>MVPISPIETVPVKLKPGMDGPKVKQWPLTEEKIKALVEICTEMEKEGKISKIGPENPYNTPVFAIKKKDSTKWRKLVDFRELNKRTQDFWEVQLGIPHPAGLKKKKSVTVLDVGDAYFSVPLDEDFRKYTAFTIPSINNETPGIRYQYNVLPQGWKGSPAIFQSSMTKILEPFKKQNPDIVIYQYMDDLYVGSDLEIGQHRTKIEELRQHLLRWGLTTPDKKHQKEPPFLWMGYELHPDKWTVQPIVLPEKDSWTVNDIQKLVGKLNWASQIYPGIKVRQLCKLLRGTKALTEVIPLTEEAELELAENREILKEPVHGVYYDPSKDLIAEIQKQGQGQWTYQIYQEPFKNLKTGKYARMRGAHTNDVKQLTEAVQKITTESIVIWGKTPKFKLPIQKETWETWWTEYWQATWIPEWEFVNTPPLVKLWYQLEKEPIVGAETFYVDGAANRE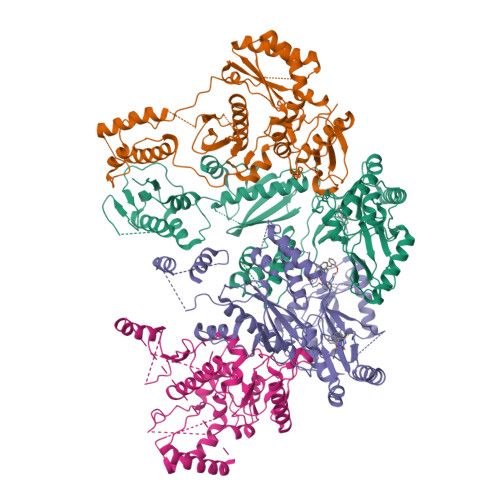TKLGKAGYVTNKGRQKVVPLTNTTNQKTELQAIYLALQDSGLEVNIVTDSQYALGIIQAQPDKSESELVNQIIEQLIKKEKVYLAWVPAHKGIGGNEQVDKLVSAGENLYFQ[4x]>MRINHNIAALNTLNRLSSNNSASQKNMEKLSSGLRINRAGDDAAGLAISEKMRGQIRGLEMASKNSQDGISLIQTAEGALTETHAILQRVRELVVQAGNTGTQDKATDLQSIQDEISALTDEIDGISNRTEFNGKKLLDGTYKVDTATPANQKNLVFQIGANATQQISVNIEDMGADALGIKEADGSIAA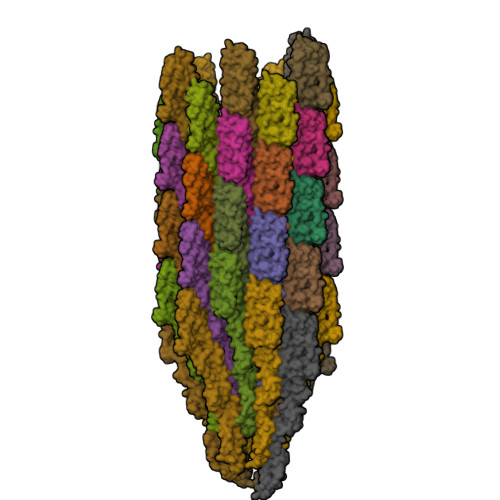LHSVNDLDVTKFADNAADCADIGFDAQLKVVDEAINQVSSQRVKLGAVQNRLEHTINNLSASGENLTAAESRIRDVDMAKEMSEFTKNNILSQASQAMLAQANQQPQNVLQLLR[46x]>[2x]GMADEATRRVVSEIPVLKTNAGPRDRELWVQRLKEEYQSLIRYVE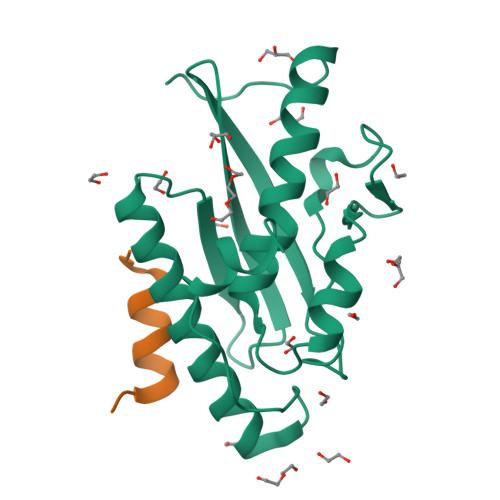NNKNADNDWFRLESNKEGTRWFGKCWYIHDLLKYEFDIEFDIPITYPTTAPEIAVPELDGKTAKMYRGGKICLTDHFKPLWARNVPKFGLAHLMALGLGPWLAVEIPDLIQKGVIQHKEKCNQ;>DSGESLEDLMAKMKNM[2x]> GMGQQESTLGG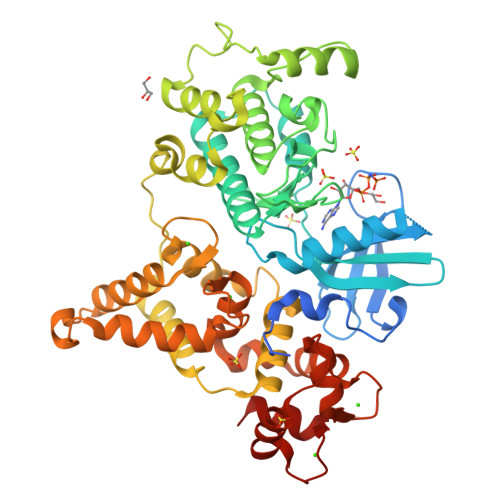AAGEPRSRGHAAGTSGGPGDHLHATPGMFVQHSTAIFSDRYKGQRVLGKGSFGEVILCKDKITGQECAVKVISKRQVKQKTDKESLLREVQLLKQLDHPNIMKLYEFFEDKGYFYLVGEVYTGGELFDEIISRKRFSEVDAARIIRQVLSGITYMHKNKIVHRDLKPENLLLESKSKDANIRIIDFGLSTHFEASKKMKDKIGTAYYIAPEVLHGTYDEKCDVWSTGVILYILLSGCPPFNGANEYDILKKVEKGKYTFELPQWKKVSESAKDLIRKMLTYVPSMRISARDALDHEWIQTYTKEQISVDVPSLDNAILNIRQFQGTQKLAQAALLYMGSKLTSQDETKELTAIFHKMDKNGDGQLDRAELIEGYKELMRMKGQDASMLDASAVEHEVDQVLDAVDFDKNGYIEYSEFVTVAMDRKTLLSRERLERAFRMFDSDNSGKISSTELATIFGVSDVDSETWKSVLSEVDKNNDGEVDFDEFQQMLLKLCGN HYDROXYPYRROLE-IMIDAZOLE-PYRROLE POLYAMIDE | C31 H41 N11 O6 | 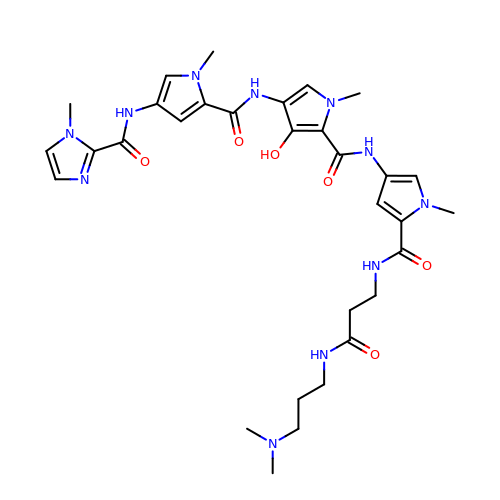WNWMZSNXDXZKBO-UHFFFAOYSA-N>MKKTSRKVVIVGTGFVGTSIAYAMINQGVANELVLIDVNQEKAEGEALDLLDGMAWGEKNVSVWSGTYEECQDANLVILTAGVNQKPGQTRLD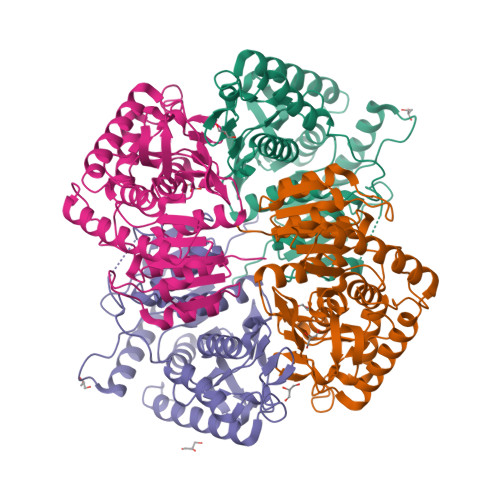LVKTNATITRQIVKEVMASGFDGIFVVASNPVDILTYLTWQESGLPASRVVGTGTTLDTTRFRKEIALKLAVDPRSVHGYILGEHGDSEVAAWSHTTVGGKPIMEYVEKDHRLEENDLTVLADKVKNAAYEIIDRKKATYYGIGMSTTRIVKAILNNEQAVLPVSAYLNGEYGEEDIFTGVPSIVDENGVREIIDLSITPQEKAMFHQSVSELKAVLDTVRLEHHHHHH[4x]> GEATTIWGVGADEAIDKGTPSKNDLQNMSADLAKNGFKGHQGVACST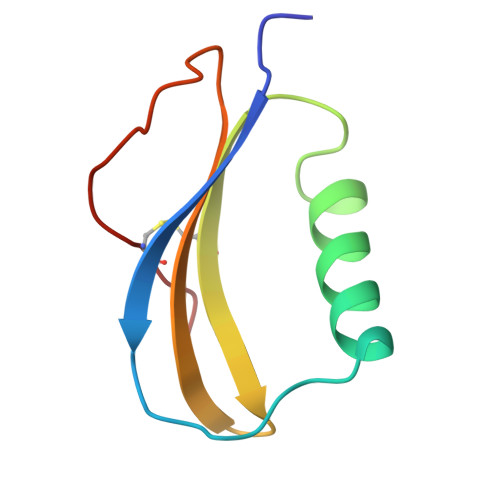VKDGNKDVYMIKFSLAGGSNDPGGSPCSDD5-AMINO-2-METHYL-6H-OXAZOLO[5,4-D]PYRIMIDIN-7-ONE 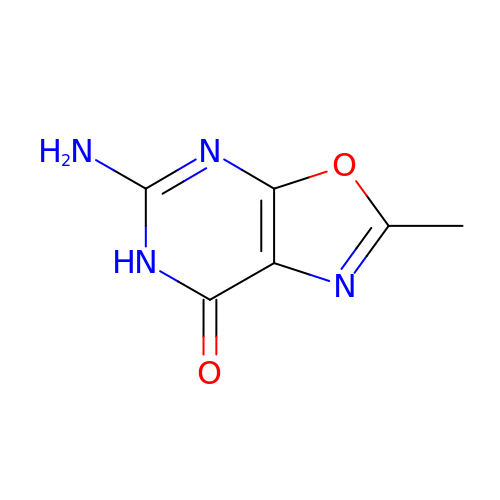| C6 H6 N4 O2 | NEKSCFHMQPOHBF-UHFFFAOYSA-N>MARTAEYSIKGYLYQFLKYLSEILAAGDGARITIEGAIEDVDVIAAGLTTAVQCKYHEQAEKYTLGKIYKPILLMLEHFSKNSGTDLHVSYRLFCHFPGESGTKALTKDDLETVLSTKGEVLRAIVARIDTSVDYEAFLDRFAIEFGPSAEDLQVAVLASLKDKGFDPDDIDAVIFPNAIQRIVDLATRSDVNDRTVEPKTFLAGLREVRRVTFTRWTRELATKGRMFSSLRKSLRSCLAHNSRWRVFVINPLTIENFDDDIVRFIKAFVQRYSSKYLHSNPPLFMLTGDYDLSVLQKRLYDAGLRCETGKVGGTDVIIKELFRRPILIRNPFRMEFSLRLAKRDEVIGGPQRRPDELFLINVADDEWKHEDVNVHGFKIERLSDLEYILQLRSDYA[12x];>[6x]MPDLGTPIGSVTDSSPSLIRIEISSAEDFEKYKSMLGVGQYLLVASGNNLYLLASITGVRATHVERRSLGPSSEVHSEEGSDGISGNFRFQIDTQPIGTLSEDGEFSRGSHSLPVPTEYAYVTPPAVLEGIFSHQIKSPFALGTLGISPDIKLKIDGDRFFSKHVAVVGSTGSGKSCAVAKILQTAVGIESKANAHKAAQKNSHIVIFDIHAEYAAAFNLEAGEAFTLNLLGVDNLRLPYWLMNAQELEQIFIESNEHNSHNQISQFRHAVVRNKCKHNPTLTNLSFDTPVYFSIDEVVTYLENMNNEVIGKLAGEGKPKLANETLVSDRDELYFDAVQSFIVASQAAATKASNGPFNGEFDRMILRLHTRLADPRLQFLFYPKKEDGEDLATGDFADVVRQFVGYMTKSNVSIIDLSGIPFEVLSIVVSLISRMIFDFGFHYSKNRHVGGAVSDVPILVVCEEAHNYLPRSGGAAYDASRKSIERIAK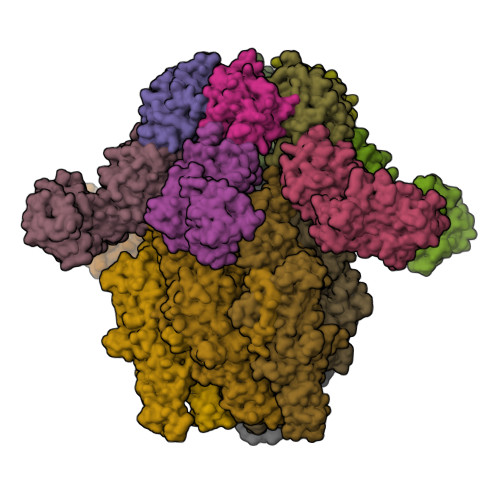EGRKYGVTLMVVSQRPSEVSETIFSQCSNFISLRLTNAVDQTYVKSLLPDLSAGLGDLLPNLAQGEFLIVGDAPLMPTVGHFALPVPEPHSRSVNYLQEWNSGWRHVDFDSVIDRWRGKVLTKSEKGV>[4x]EVPQMTSSSAPDLEEEDDYTAYAPLTCYFTN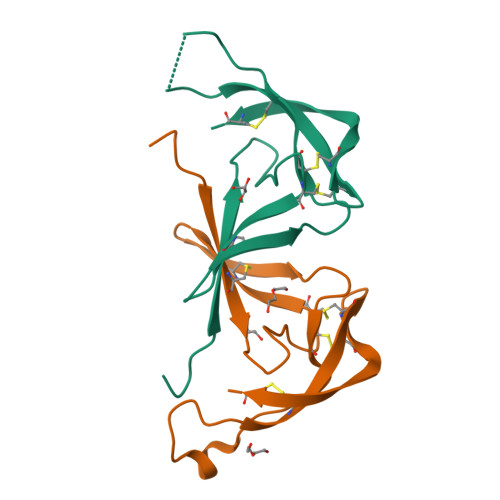STLGLLAPPNCSVLCNSTTTWFNETSPNNASCLLTVDFLTQDAILQENQPYNCSVGHCDNGTCAGPPRHAQCW>[33x]MAINVNTNVSAMTAQRYLNGAADGMQKSMERLSSGYKINSARDDAAGLQISNRLTSQSRGLDMAVKNANDGISIAQTAEGAMNET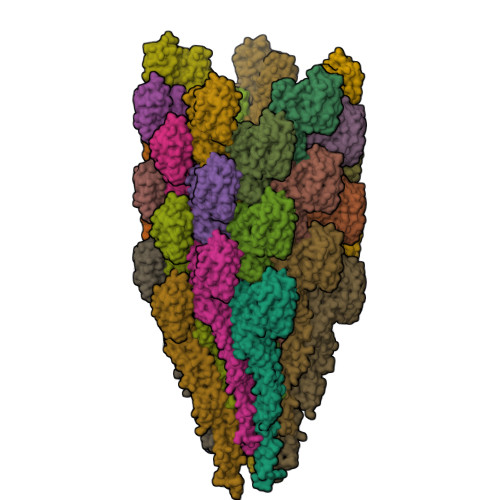TNILQRMRDLALQSSNGSNSSSERRAIQEEVSALNDELNRIAETTSFGGNKLLNGSFGSKSFQIGADSGEAVMLSMGSMRSDTQAMGGKSYRAQEGKAADWRVGAATDLTLSYTNKQGEAREVTINAKQGDDLEELATYINGQTEDVKASVGEDGKLQLFASSQKVNGDVTIGGGLGGEIGFDAGRNVTVADVNVSTVAGSQEAVSILDGALKAVDSQRASLGAFQNRFGHAISNLDNVNENVNASRSRIRDTDYARETTAMTKAQILQQASTSVLAQAKQSPSAALSLLG>[7x]XGEIAKALREIAKALRE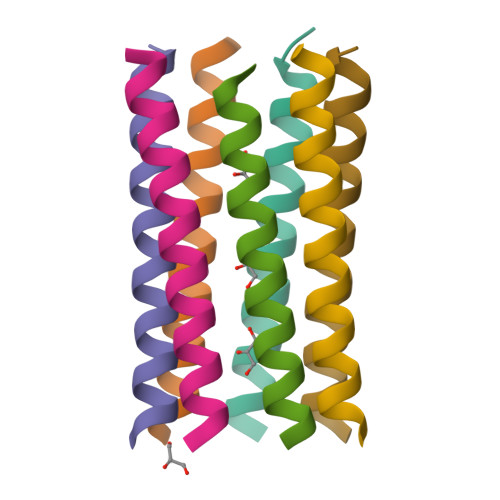IAWALREEAKALRGX>[3x]GDTSPAQLIAGYEAAAGAPADAERGRALFLSTQTGGKP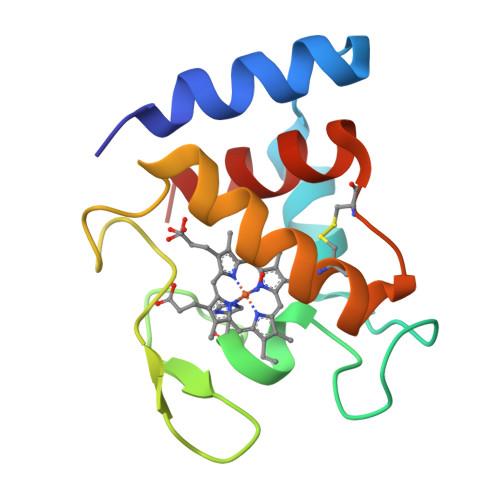DTPSCTTCHGADVTRAGQTRTGKEIAPLAPSATPDRFTDSARVEKWLGRNCNSVIGRDCTPGEKADLLAWLAAQ> MEEVFQNETIKQILAKYRRIWAIGHAQSVLGWDLEVNMPKEGILERSVAQGELSVLSHELLLHPEFVNLVEKAKGLENLNEYERGIVRVLDRSIRIARAFPPEFIREVSETTSLATKAWEEAKAKDDFSKFEPWLDKIISLAKRAAEYLGYEEEPYDALLDLYEEGLRTRDVEKMFEVLEKKLKPLLDKILEEGKVPREHPLEKEKYEREWMERVNLWILQKFGFPLGTRARLDVSAHPFTTEFGIRDVRITTRYEGYDFRRTILSTVHEFGHALYELQQDERFMFTPIAGGVSLGIHESQSRFWENIIGRSKEFVELIYPVLKENLPFMSNYTPEDVYLYFNIVRPDFIRTEADVVTYNFHILLRFKLERLMVSEEIKAKDLPEMWNDEMERLLGIRPRKYSEGILQDIHWAHGSIGYFPTYTIGTLLSAQLYYHIKKDIPDFEEKVAKAEFDPIKAWLREKIHRWGSIYPPKELLK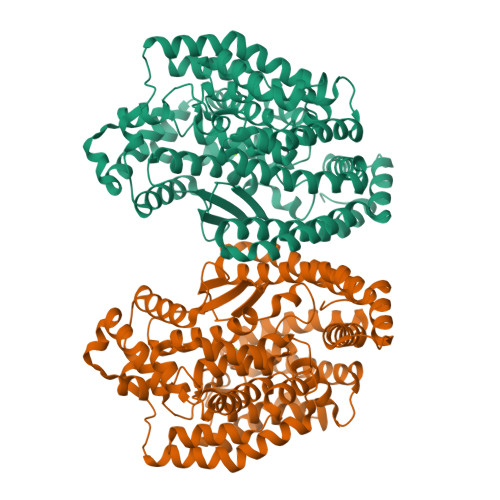KAIGEDMDAEYFVRWVKEKYL> VRLPGLAAMRQGTRLFTPEQGEDLREALRRRRGSFQTTCEVTSETTFAAARRLREKASALAALNFASAKNPGGGFLGGAQAQEEDLCRGSGLYFSLTSPQAEPYYAVNRQSHSALYTDHLIYSPQVPIFRDDAGQLLPAPVPVNIITAPAPNAGAVAQSRPEQLPQVLPTLRERARRVLGVAAWMEQTHLVLGAWGCGVFRNDPAGVARTFRELLEGEAQGAFEHVTFAVLDNHPQHPTLGAFRRELESLC

Despite the abundance of PARP1, most of the PAR generated by DNA damage is rapidly degraded, with a half-life of less than 1 min by poly (ADP-ribose) glycohydrolase (PARG). The radio-resistant bacterium D. radiodurans encodes a PARG homolog, DrPARG, whose expression is upregulated after radiation damage, so it might play an important role in DNA repair. Our study demonstrates that DrPARG is involved in catalyzing the breakdown of endogenous PAR and DNA repair in D. radiodurans. From observing the structural peculiarities of DrPARG, we show that although previously thought to be an obligate exo-glycohydrolase, bacterial PARG could exert both exo- and endo-glycohydrolase functions.

Therefore, we attempted to obtain crystals of DrPARG in complex with ADP-ribose. Crystals were found in several similar conditions, but they belonged to different space groups. Notably, the 28 N-terminal residues of these solved structures from different space groups, including P21, P32, P3221, and P212121, were not well defined in the electron density maps, which suggests that this phenomenon did not result from crystal packing. In fact, the missing residues located in the intrinsically disordered N-terminal region of DrPARG and might be highly flexible. The structural flexibility may reflect the multiple space groups observed in X-ray crystallography because packing patterns are constantly influenced by the flexible regions during crystallization.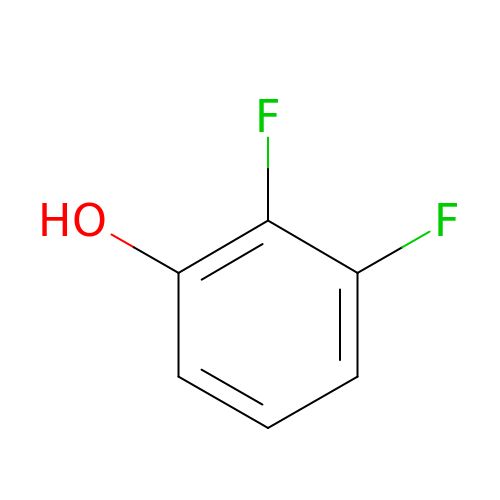2,3-bis(fluoranyl)phenol | C6 H4 F2 O | RPEPGIOVXBBUMJ-UHFFFAOYSA-N>[4x]MGSQRTTAVKGERQSRVHTGNPHPTLTYDI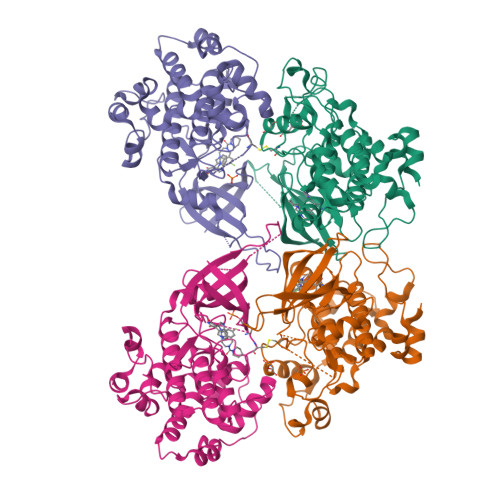GRVLGNGSFGVVTEARCVDTGEVVAIKKVLQDPRYKNRELDIMKELKHPNVVKLIDYFYTEMGERDSNDHNRFLNVVMEHIPETVYRVMKSFLRANQQVPFILIKLYTYQMCRALGYLHALGICHRDIKPQNLLVDSRTHVLKLCDFGSAKRLVPGEQSVSYICSRFYRAPELMLGASEYTTAIDVWSIGCVLGELLLGRPLFAGETSVDQLVKIIQILGTPSRRQMSTMNPNYTEFRFPDVKPREWKSIFASHIASTETNDPSWDQALDLLTKFLRYEPGERLLPLEALAHDFFDELRLPSTRLPSGGPLPELFTFSQLELQNMSPAAQVKCIPKGHHHHHH>MKSSHHHHHHENLYFQSNAEESAQQRSERYVSARSQHPAWLLLASRRAPLVLGCLRTLFERAHDGIPMEDALQALSEMLAAYASQELYEIDPDATHLQAGRELREWIKRRLVVEREGRIYATDALESAIQFVDSLDSRIMTSTASRLSVVQREIENLETGLNPSPTGRIASLRRRIQDLEHELARVEAGHVDVLDEAQAIEGMREVYNLATSLRADFRRVEDSWREADRALRHSIISEQSHRGEIVDRLLDGQDALLNTPEGRVFESFQQQLRQSAELEVMRERLRTILRHPAVPKALNRPQQRELRWLALRLVRESQAVLQARARSERDVRGFMKTGLAAEHHRVGQLLNDFFNLALSVDWQRQSERRKPACLPPVGVAITGVPAIERLRFKTLDDDDAGELDLSLKPAGLEQIDDDFWDAFDGLDREALIHDTLAVLVEQGRPVSLGELASLLPPAHDLETFALWLAMAREAGIEVLTEERQFVELVDEDEQRWGFNLPYVGLDHEALKDIDWEL[2x];>MKSSHHHHHHENLYFQSNAKQALLWRDSETFILTSIELYNWGGFQGYHRAEIDPSGTAVIGPTGSGKTTLVDALMTLLCANPRYNLASTGGHESDRDLVSYVRGVTGPGDGGVEQSHIARQGKTVTAIAATLERDGAQVRLGAVLWFEGTSSSASDLKKLWLLSESPEQTLEHWLSQHHAGGMRALRQMEKDGMGIWPYPSKKAFLARLRDYFEVGENAFTLLNRAAGLKQLNSIDEIFRELVLDDRSAFERAAEVASSFDDLTDIHRELETARKQQRSLQPVADGWERYRALQEQLQDKQALEGILPVWFAEQGYRLWLAETNRLEKEHKQAELDQAQCRSQLEIQKGVVDQHRQRYLRVGGAGIDQLRGRIADWVRECDKRRLKAEQYQRLAKGLGLADELSAAALEENQQQIAARLEILAQQTTDARQKAFDAGLVQQELNGRLQSLQQERAEVERRPGSNLPGHFHAFRGDLAQELGVDESALPFVAELVQVKPEELAWRGAIERAIGSHRLRILVPQGSSQAALRWVNQRH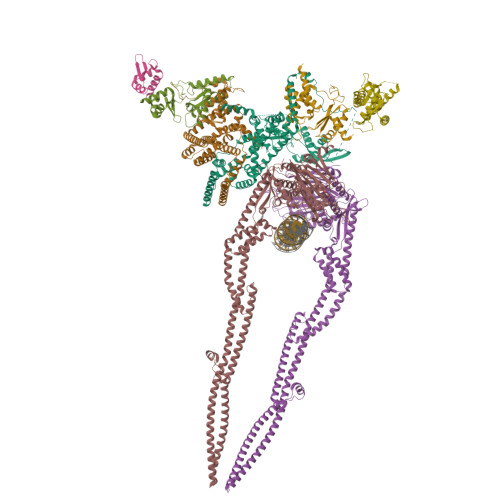NRLHVRLLEVKEPSSRPVFFDDGFTRKLTFKEHPYREAVKALLADNDRHCVESTEQLRHTPHAMTAQGLMSGKERFFDKQDQKRLDEDWLTGFDNRDRLAFLAEQIREVNEQLVPAKLALDAAQGDVGQLESQASLLQRIEELQFDDIDRPGAERQLQSLRTQLDTLTRPDSNLAVIKAELDQAEALRESLDQQLQRLIEQCVQLKTQFDQAASATRKAYRGAEKGLSDTQRELAQAHFPILSTDDLGDIDELERKHTRELQGQLKTLGEKLGDQKTELAKRMSDALKADTGALAEVGRELVDVPRYLERLRVLTEEALPEKLKRFLEYLNRSSDDGVTQLLSYIDHEVSMIEERLDDLNSTMQRVDFQPGRYLRLVAKKVIHESLRTLQHAQRQLNSARFIDDEGESHYKALQALVGLLKDACEHSRNQGAKALLDPRFRLEFAVSVIDREGNNLIETRTGSQGGSGGEKEIIASYVLTASLSYALCPDGSSRPLFGTIVLDQAFSRSSHAVAGRIIAALREFGLHAVFITPNKEMRLLRHHTRSAVVVHRRGVESSLVSLSWEALDEHHQQRIRAMHEVAH[2x];>[4x]MAGIFDRIAGASGADETELTAEPMALDDGMDGEQPAMSANIQVDERRTPQRVREAVQEMLKYGLLEESHKPNLYRSALTNIEVVDRILEPLDLAMGVDEVRGLVFVTVRQGEVAEQDDWSHPLVRRQRLNLEQSLLIAILRQHFIAYEQESGTGASQALVAVDELIPQLQVYLGELGSEAKERNRIITLLDQLKGHGLVSALDAHDRVIIRPIITHLANPENLQALVVWLREQVEGAVTPAAGGEEDEA>DADLWSSHDKMLAQPLKDSDVEVYNIIKKESNRQRVGLELIASENFASRAVLEALGSCLNNKYSEGYPGQRYYGGTEFIDELETLCQKRALQAYKLDPQCWGVNVQPYSGSPANFAVYTALVEPNGAIMGLDLPDGGHLTHGFMTDKKKISATSIFFNSMPYKVNPDTGYINYDQLEENARLFHPKLIIAGTSCYSRNLEYARLRKIADENGAYLMADMAHISGLVAAGVVPSPFEHCHVVTTTTHKTLRGCRAGMIFYRKGVKSVDPKTGKEILYNLESLINSAVFPGLQGGPHNHAIAGVAVALKQAMTLEFKVYQHQVVANCRALSEALTELGY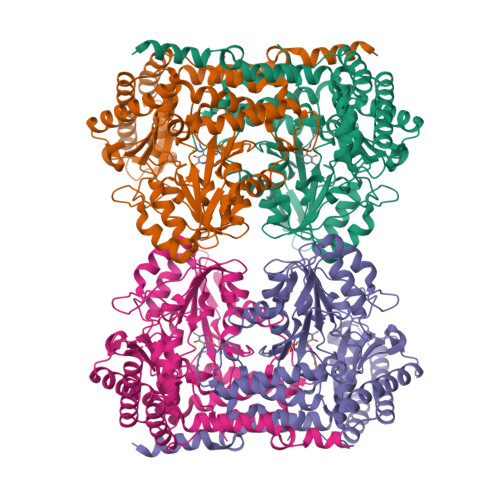KIVTGGSDNHLILVDLRSKGTDGGRAEKVLEACSIACNKNTCPGDRSALRPSGLRLGTPALTSRGLLEKDFQKVAHFIHRGIELTLQIQSDTGVRATLKEFKERLAGDKYQAAVQALREEVESFASLFPLPGLP[4x]5-fluoranyl-2-[5-[[1-(1-methylpiperidin-4-yl)pyrazol-4-yl]amino]-[1,2,3]triazolo[4,5-d]pyrimidin-3-yl]benzenecarbonitrile | C20 H19 F N10 | 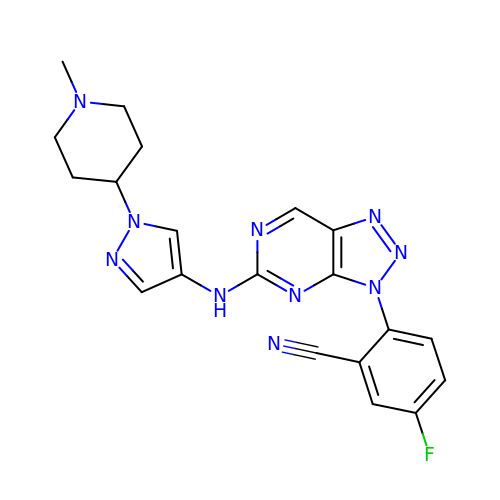AWEOBSGKFWBFJW-UHFFFAOYSA-N> MSEFVSIAARQEGAVGIIELARPDVLNALSRQMVAEIVAAVEAFDRNEKVRVIVLTGRGRAFAAGADIQEMAKDDPIRLEWLNQFADWDRLSIVKTPMIAAVNGLALGGGFELALSCDLIVASSAAEFGFPEVNLGVMPGAGGTQRLTKLIGPKRALEWLWTGARMSAKEAEQLGIVNRVVSPELLMEETMRLAGRLAEQPPLALRLIKEAVQKAVDYPLYEGMQFERKNFYLLFASEDQKEGMAAFLEKRKPRFQG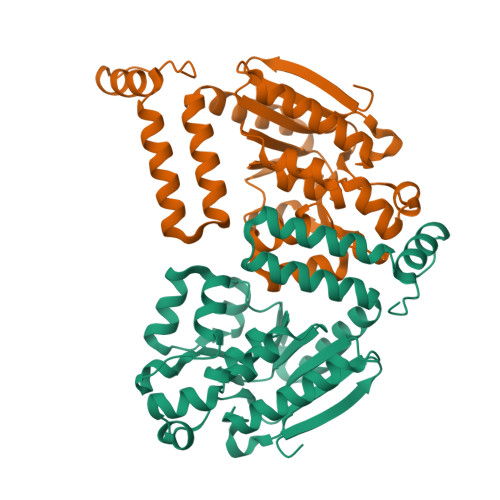K>AEGDDPAKAAFNSLQASATEYIGYAWAM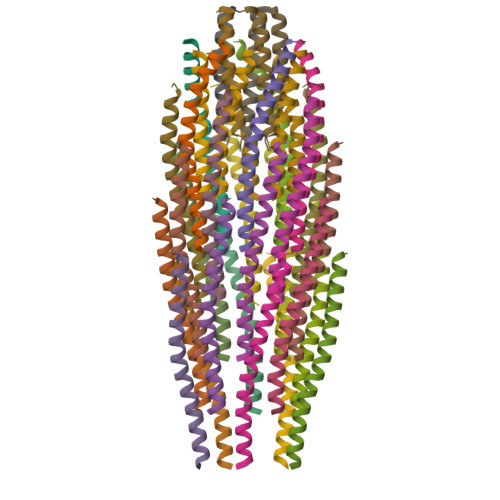VVVIVGATIGIKLFKKFTSKAS[25x];>[5x]MEQVADFDTIYQAMIQISVVLCFALGIIAGGQR;>MSVLVYSFASFVLGWCLRSGITYFTRLMETSS[5x]>MHHHHHHENLYFQGAASMKAYLVGLYTLTPTHPGSGTELGVVDQPIQRERHTGFPVIWGQSLKGVLRSYLKLVEKVDEEKINKIFGPPTEKAHEQAGLISVGDAKILFFPVRSLKGVYAYVTSPLVLNRFKRDLELAGVKNFQTEIPELTDTAIASEEITVDNKVILEEFAILIQKDDKGILESVVKAIEQAFGNEMAEKIKGRIAIIPDDVFRDLVELSTEIVARIRINAETGTVETGGLWYEEYIPSDTLFYSLILVTPRAKDND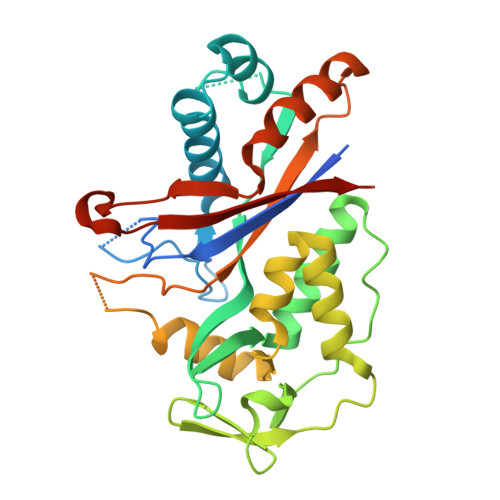MALIKEVLGKINGKYLQIGGNETVGKGFVKVTLKEVTNNGGTHAK[4x]>GSHMVPISFVFNRFPRMVRDLAKKMNKEVNFIMRGEDTELDRTFVEEIGEPLLHLLRNAIDHGIEPKEERIAKGKPPIGTLILSARHEGNNVVIEVEDDGRGIDKEKIIRKAIEKGLIDESKAATLSDQEILNFLFVPGFSTKEKVSEVSGRGVGMDVVKNVVESLNGSISIESEKDKGTKVTIRLPLTLAIIQALLVKVNNLVYAIPIANIDTILSISKEDIQRVQDRDVIVIRGEVIPVYRLWEVLQIEHKEELEEMEAVIVRVGNRKYGIVVDDLLGQDDIVIKSLGKVFSEVKEFSGAAILGDGSIALIINVSGIV[2x];>MKTLADALKEFEVLSFEIDEQALAFDVDNIEMVIEKSDITPVPKSRHFVEGVINLRGRIIPVVNLAKILGISFDEQKMKSIIVARTKDVEVGFLVDRVL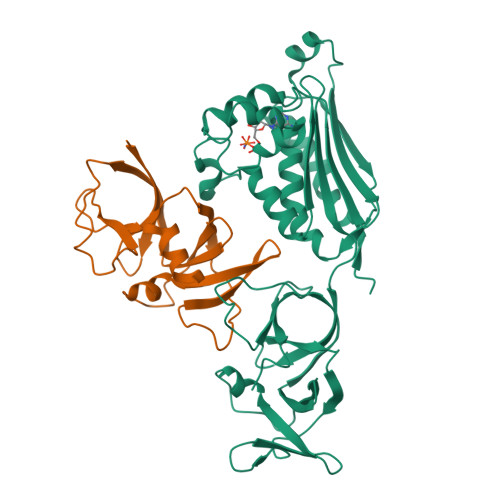GVLRITENQLDLTNVSDKFGKKSKGLVKTDGRLIIYLDIDKIIEEITVKEGV[2x]> MATSNVVVSRTGTGWTVDVTACNLLSDTGIKDFIVLHNAIVVSNVTYAKTTATTLTYTGAALPSNTPVEIRRKTPNSIIQLVTYGQKLSSNLWNSEIDRNIRWREEVDLNGAGLVASTPTPQNDAYGLVWAGDTFYPPTRKSVYDKIETLATKSGAVLTGATANVSPSTADNTLALA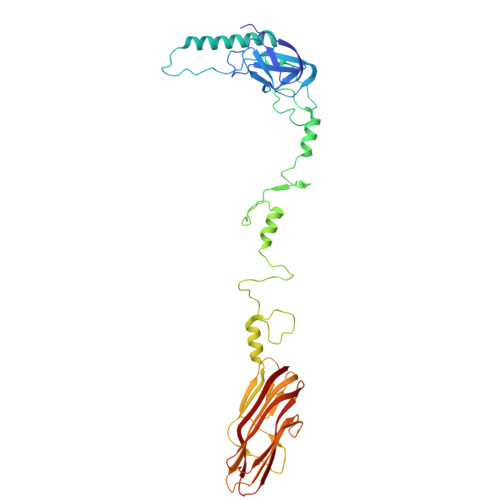TTAYVKANLADYATLVSPILTGDPRAVTTSVTDNDTSIATTAHVRAFANSRLAFNAFRGGQQGVPSLNYITTVCQFTSSAVRSGWGDNFSSNRWLVGQGGTYYVSVTCRFATTGGTPPTYMDVLLFVGLSPTGVENFVIRQQTNYPSFGYTLTWSGVLFFNTNDNVYLTYQAQAIGGGGYAVVIEDARFNAIQLS> LIKGPWTKEEDQRVIKLVQKYGPKRWSVIAKHLKGRIG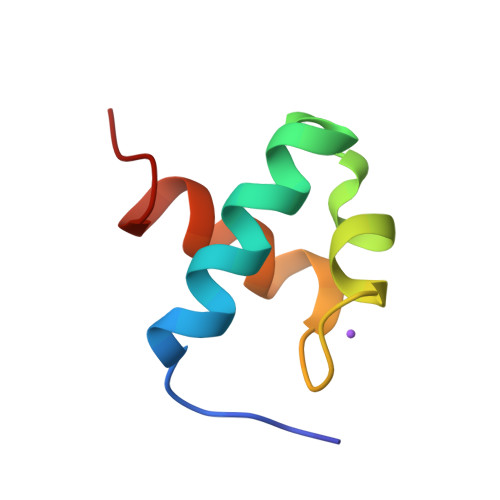KQCRERWHNHLNPE> NTDLAIQGNGFFILKDGEKTFYTRAGAFGIDKEGTLVNPANGMRVQGWMAEEAEGFRIINTSGQTEDLNIPIGQKLDAKATTSVNYAANLDKRLPELPEGANRAQILESTWSTEFKVYDSFGEAHELQIDFARVPGEVNAWRATVNVD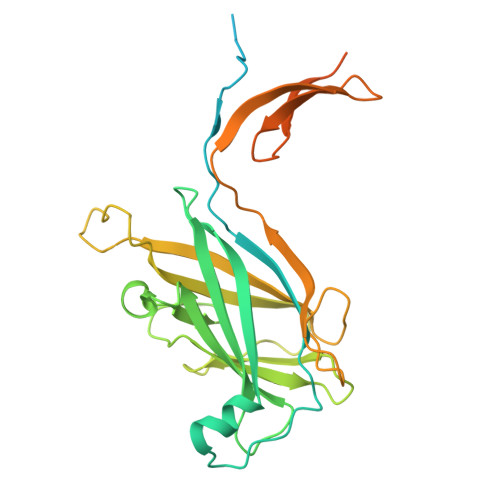PTNADATATRVGIGTTDGVQNSFIVRFDNNGHLASVTDTAGNVTSPAGQVLVQISYNVVGANPDEAGAPTRHTFDVNLGEIGTSKNTITQFSDKSTTKAYEQDGYTLGYLENFRIDQSGIITGVYSNGVRQEIGQIAMAGFANQGGLEKAGQNTYVQSNNSGIANVSTSGTVGKGYFIGGTLEMS6-{3-[(1-methyl-1H-imidazol-2-yl)sulfanyl]phenyl}pyridin-2(1H)-one | C15 H13 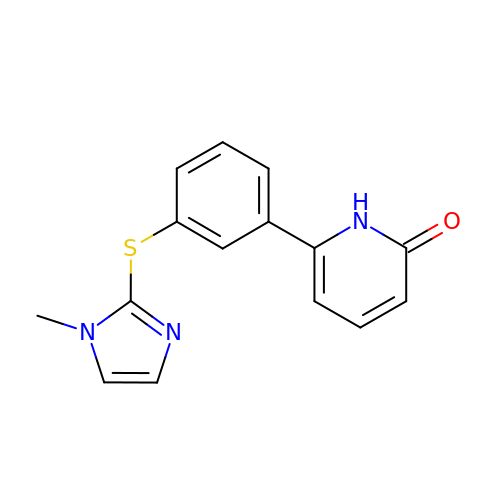N3 O S | YYWBGPHQPMDZEM-UHFFFAOYSA-N>[4x]QEESILQDIITRFPNVVLMKQT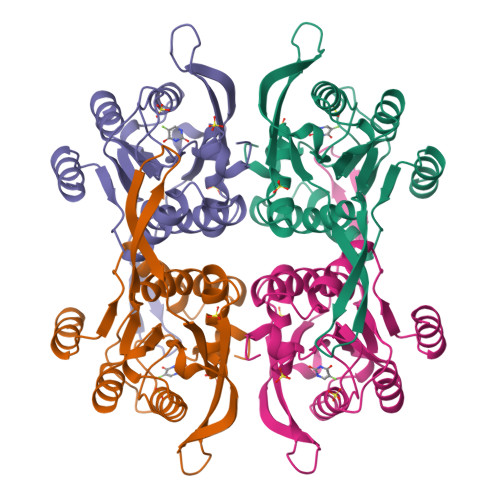AQLRAMMTIIRDKETPKEEFVFYADRLIRLLIEEALNELPFQKKEVTTPLDVSYHGVSFYSKICGVSIVRAGESMESGLRAVCRGVRIGKILIQRDETTAEPKLIYEKLPADIRERWVMLLDPMCATAGSVCKAIEVLLRLGVKEERIIFVNILAAPQGIERVFKEYPKVRMVTAAVDICLNSRYYIVPGIGDFGDRYFGTM Nalpha-(2-fluoro-4-{4-[4-(trifluoromethyl)phenyl]piperazin-1-yl}benzoyl)-N-pyridin-4-yl-D-tryptophanamide | C34 H30 F4 N6 O2 | 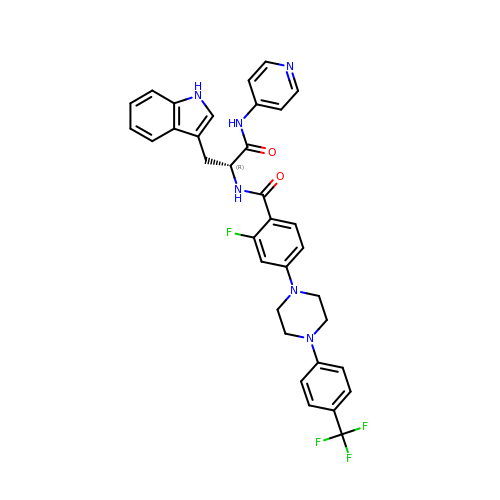CYPNHMRAJORLFS-WJOKGBTCSA-N(2R)-2-ethyl-4-hydroxy-5-methylfuran-3(2H)-one 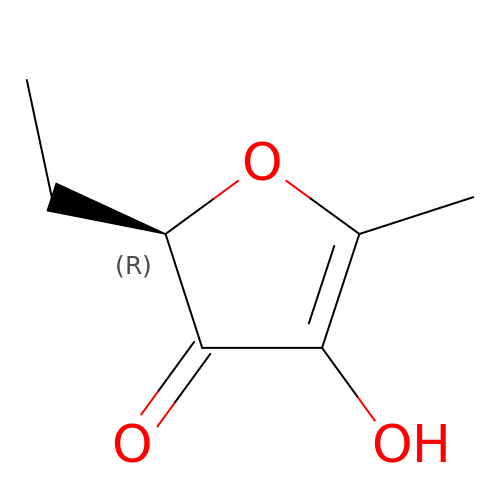| C7 H10 O3 | GWCRPYGYVRXVLI-RXMQYKEDSA-N>MGYLNREERRETIMQAAMRVALDQGFTGMTVRNIATAAGVAAGQVHHHFTSSGELKSQAFIRVIREMMDLQRLSRTAGWREQLFSALGSEDGRL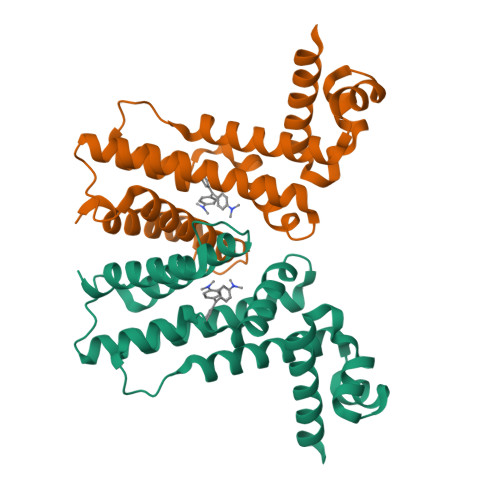EPYIRLWRQAQLLADSDPEIKSAYLLTMNLWHDEAVRIIRAGHAAGEFTLRDSAENIAWRLISLVCGLDGIYVLGMPEVDDAAFTRHLQHVIQLELFS[8x]5-[({3-hydroxy-2-methyl-5-[(phosphonooxy)methyl]pyridin-4-yl}methyl)amino]pentanoic acid | C13 H21 N2 O7 P | 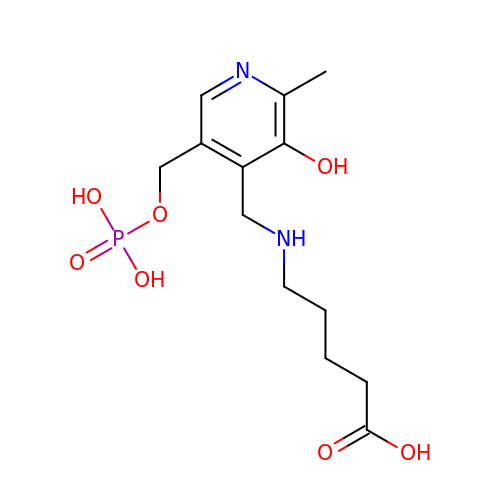JXMZQLZPXCDFBY-UHFFFAOYSA-N> YEIIRTNVQEVLAEIVSPSTKNPNSENPAVKKRFRGIKNVVSRIISNDKKCRYDLIYNKYLSSSDTRKLKTMIDYSTKFNRVVEVVLIIMGKLLPLDAWGGTENKKVIQDRIVDFLRLGANERLHLDDVLSGIKLSKFKWLGVGNNISSQQDFQIRKRLLEGYINWVFISLVKNIVRAFWYVTESSNMDCSKLFYFTHSIWNELSSNWITKYAKGNLVQVVSPESKGQFTNGKIKLIPKRGGFRVICVPLKQSLYSFNN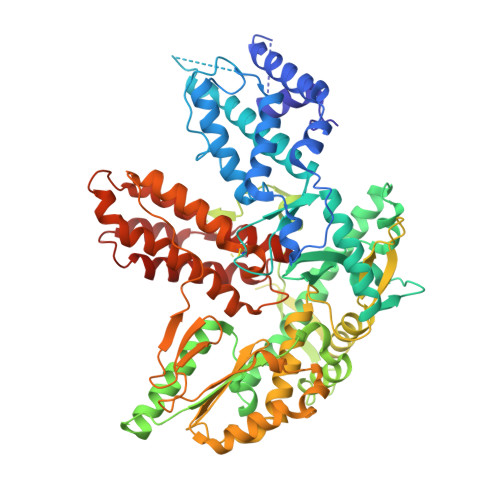KRNFALKQKEKWDYIFYQKYTLSPVRQVLQLKLNALRKSDMGHRSSVNSTNEVADRILTFRNDLLKKNKTLPVLYMIKFDMKECYDRLNQNALKESIAGIFKEDNENTTYHVREYGTLDEFLKLKRVRTLIETEVQNFNIIMNSKDEAEAGSRSYGTKVDKVKTLSISKNKIIEVCHSQIEDATCLVKNKEGQYDLFKRKQGVFQGFSLSGIFCDILYSTMVSKEFKFLWEATEDNLLLRLVDDFIFITSNKDTLKKVKDKISSNELQKYGAFVNHEKTVEINGEAGSSNKMTFVGLDINCLTLDVKKDSSQFSRPTCKFRSFKALFSNLKQFYCSNLCEFLLDFSSNSLETIRENVDAILKLTFEAIQTSFATISKQDSFERYRFMKFLHVIIETTIEKFARVNGSMEGVEYLLTCIKITITKSLAFMATKQEIIEWLYTLTIVD>[4x]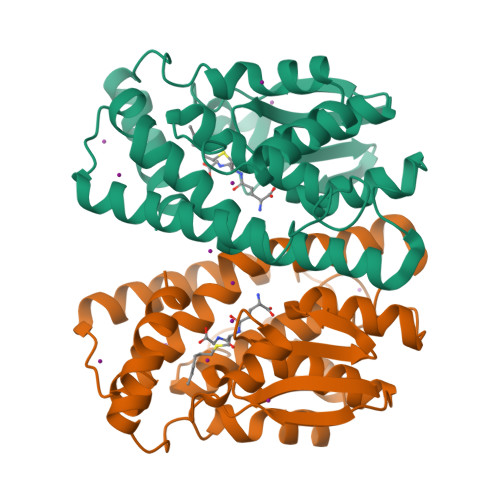MHHHHHHMGLELYLDLLSQPCRAVYIFAKKNDIPFELRIVDLIKGQHLSDAFAQVNPLKKVPALKDGDFTLTESVAILLYLTRKYKVPDYWYPQDLQARARVDEYLAWQHTTLRRSCLRALWHKVMFPVFLGEPVSPQTLAATLAELDVTLQLLEDKFLQNKAFLTGPHISLADLVAITELMHPVGAGCQVFEGRPKLATWRQRVEAAVGEDLFQEAHEVILKAKDFPPADPTIKQKLMPRVLAMIR>GSMEPAMEPETLEARINRATNPLNKELDWASINGFCEQLNEDFEGPPLATRLLAHKIQSPQEWEAIQALTVLETCMKSCGKRFHDEVGKFRFLNELIKVVSPKYLGSRTSEKVKNKILELLYSWTVGLPEEVKIAEAYQMLKKQGIVKS[2x];>[2x]SASVSLLDDELM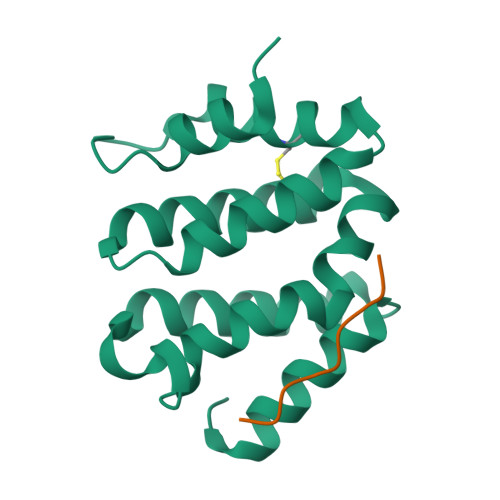SL> SPNVEACGYSDRVQQITLGNSTITTQEAANAVVCYAEWPEYLPDVDASDVNKTSKPDTSVCRFYTLDSKTWTTGSKGWCWKLPDALKDMGVFGQNMFFHSLGRSGYTVHVQCNATKFHSGCLLVVVIPEHQLASHEGGNVSVKYTFTHPGERGIDLSSANEV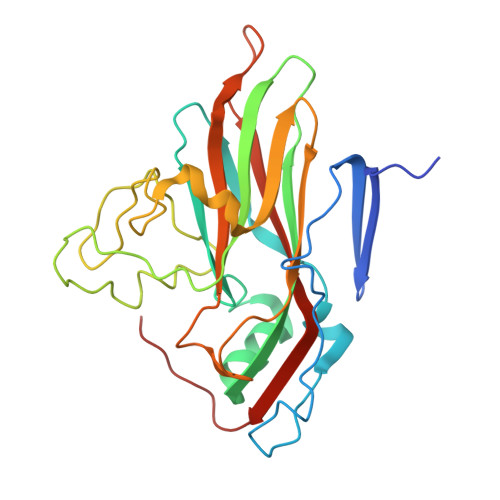GGPVKDVVYNMNGTLLGNLLIFPHQFINLRTNNTATIVIPYINSVPIDSMTRHNNVSLMVIPIAPLTVPTGATPSLPITVTIAPMCTEFSGIRSKSIVPQ>MGHHHHHHHHHHSSGHIEGRHIGSGVEAPEQLEEHGISVYATIPMSEWLDKRTRLRKKNLFSNQQRHRTKNIPFLAVDNPADSAVEAVRALRTSLHFAMMETENNILMITGATPDSGKTFVSSTLAAVIAQSDQKVLFIDADLRRGYSHNLFTVSNEHGLSEYLAGKDELNKVIQHFGKGGFDVITRGQVPPNPSELLMRDRMRQLLEWANDHYDLVIVDTPPMLAVSDAAVVGRSVGTSLLVARFGLNTAKEVSLSMQRLEQAGVNIKGAILNG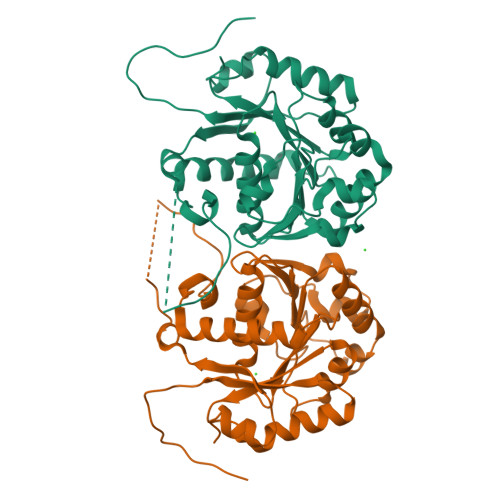VIKRASTAYSYGYNYYGYSYSEKE[2x]> GSANSQLVVRAKFNFQQTNEDELSFSKGDVIHVTRVEEGGWWEGTHNGRTGWFPSN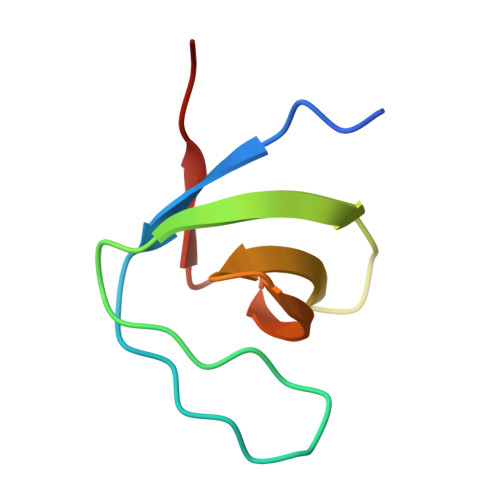YVREIKPS> AAKREDLEKKQQLLRAATGKAILNGIDSINKVLEHFRRKGINQHVQNGYHGIVMNNFECEPAFYTCVEVTAGNRLFYHIVDSDEVSTKILMEFNKMNLPGEVTFLPLNKLDVRDTAYPETNDAIPMISKLRYNPRFDKAFKHVFGKTLICRSMEVSTQLARA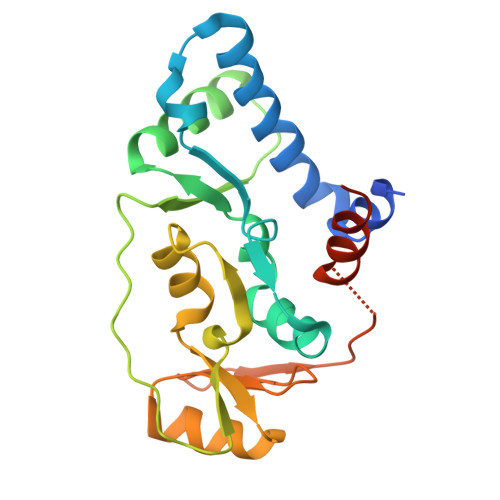FTMDCITLEGDQVSHRGALTGGYYDTRKSRLELQKDVRKAEEELGELEAKL>[4x]MHLMNMVDPDFNSLIELSKSAGDMTKIEPAMLRNFLDESSLSSRGAPVEIKEIKDYKIKLDGRTLNARMYDDNNAKSAILYYHGGGFLFGNIETYDNYCRFLAKESGVKIISIEYRLAPEHKFPDAFNDAYDSFHYIAKKKKDFGIEGRIGVAGDSAGANLAAALCLK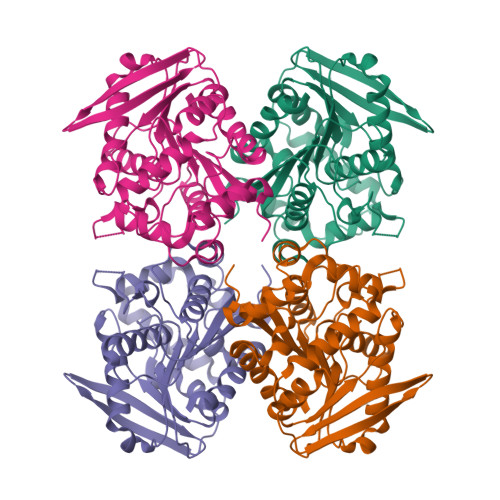CRDGKTEMPAVQVLFYPSLAPDNFSRSFIEYSDNYVLTGKMIRYFGNMYSKNMQDLINPYFSPLVADDFSNLPPAIMVTNEYDPLRDPEETYVKKLREAGVRAVGIRGIGMIHGSATDFEVSDGARNIVKMVARIIPDYL UdgX excises uracil from uracil-containing DNA to concurrently form a covalent bond with the resulting AP-DNA. Structurally, UdgX is highly similar to family-4 UDGs (F4-UDGs). However, UdgX is unique in possessing a flexible R-loop (105KRRIH109). Our earlier studies allowed us to propose a reaction mechanism of UdgX, which involves the formation of a covalent bond between H109 of UdgX with the C1′ position of the target deoxyribose sugar concurrently with the uracil excision from this site in DNA.

Furthermore, based on our structural analyses, we suggested that R184 in the DNA intercalation loop (motif B) facilitates localization of the target U in the active site. We combined H109S and R184A mutations and measured the kinetics of uracil excision. H109S/R184A mutant showed nearly 2-fold increase in its Km as compared to H109S, and about 4-fold decrease in Kcat/Km. To understand this further, we determined the structure of H109S/R184A mutant and compared the R184A region of it with the structure of UdgX–DNA complex. Nonetheless, all structures revealed the excised uracil and the side chain substitutions at position 109. The NG and NE of R184 established H-bonds of 3.53 and 3.55 Å lengths with the phosphate backbone of DNA (P + 1), and the NE of R184 makes another hydrogen bond with (P – 1) of DNA backbone with 2.32 Å distance. These observations emphasise the role of R184 in binding of DNA substrate with UdgX. In addition, our biochemical and structural analysis of the R184 mutant shows that R184 is critical in binding to the DNA by establishing multiple interactions with the phosphate backbone in the neighbourhood of the uracil in the DNA. The R184A mutation results in ∼2-fold increase in Km for DNA binding and an overall reduction of ∼4 fold in Kcat/Km value of the mutant confirming its role in stabilization of the enzyme substrate complex.

> AGAQDFVPHTADLAELAAAAGECRGCGLYRDATQAVFGAGGRSARIMMIGEQPGDKEDLAGLPFVGPAGRLLDRALEAADIDRDALYVTNAVKHFKFTRAAGGKRRISKTPSRTEVVACRPWLIAEMTSVEPDVVVLLGATAAKALLGNDFRVTQHRGEVLHVDDVPGDPALVATVHPSSLLAGPKEERESAFAGLVDDLRVAADV> GSSVTVRPDWVTIEEMDFPRLSKLTLPGVKEGEDVLCCGAVEYYDKSYDRVNVKNEKPLQRIDRIFHTVTTTDDPVIRKLSKTEGNVYATDAILATIMCCTRSNYSWDIVIEKIGNKLFFDKRDNTEFDLLTVNETSVEPPQDDGNSLNSPRNLALEATFINHNFSQQVLKSNEPRYKFDEPNPFISEEEEGEVASVAYRYRKWDLNNGITLIARCEHDAVMQGP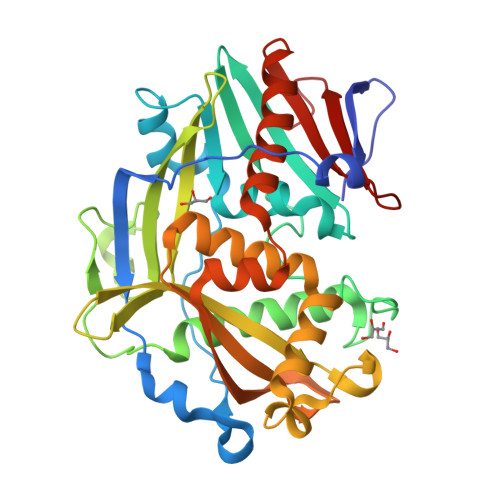NNETQFLTIKALNEWDSKLANGVEWRRKLDTQRGAVLANELRNNACKLAKWTVQALLAGSDQLKFGYVSRASVRDSSKHVILETQQYKPNEFATQINLNMDNAWGILRCIIDICMNQKDGKYLIMKDPNKPMIRLYDIPDNTF The membrane-bound EssB is an integral and essential component of the bacterial type VII secretion system that can contribute to pathogenicity. One of these is EssB, a 50-kDa bitopic integral membrane protein that is conserved among T7SS gene clusters in Firmicutes. The architecture of Geobacillus thermodenitrificans EssB has been investigated by combining crystallographic and EPR spectroscopic methods. The protein forms a dimer that straddles the cytoplasmic membrane.

We determined the crystal structure of EssB-N using a construct comprising the entire predicted cytoplasmic fragment (Ser2 to Asp214). The structure of EssB-N was determined at 1.7 Å resolution. The asymmetric unit consists of a single polypeptide folded into an elongated structure, approximately 55 Å long and 35 Å wide, which consists of two domains. The N-terminal domain is dominated by a four-stranded antiparallel β sheet. The C-terminal domain consists of a helical bundle formed by two antiparallel helix pairs, α4/α5 and α7/α8. A cleft, approximately 30 Å deep, is formed between the two domains, blocked at one side by the interdomain connecting loop that links β4 to β5. The EssB-N segment resembles the bilobal structure of ATP-dependent protein kinases, i.e., an N-terminal domain or N-lobe with a β sheet packed against an intersecting α-helix, and a predominantly α-helical C-terminal domain (C-lobe; Zoltner et al., 2013). An overlay provides a Z-score of 10.4 and a root-mean-square deviation (rmsd) of 4.4 Å for an alignment of 173 Cα-atoms. These values suggest a distant evolutionary relationship but the catalytic residues are absent from EssB-N. However, at the C-terminal inner surface of the EssB cleft, as well as at the domain contact area, a remarkable degree of structural similarity is evident (Zoltner et al., 2013). The transition to a monomeric state appears to be influenced by a combination of low pH and high ionic strength, which matches the crystallization conditions used for EssB-N where we may have been selecting out the monomer.

> GASTSEKKTYLETQLDAVMINDQPYTVIFQRAKLKMQDPLELEVLKEVDPCIVRDIDVSEDEVKVVIKPPSSFLTFAAIRKTTLLSRIRAAIHLVSKVKHHSARRLIFIVCPENLMFNRALEPFFLHVGVKESLPPDEWDDERLLREVKATVLALTEGEYRFDEYLKFHETLKCSPIAKELWQADHLDAVLAVLEKWVDEEEAKERAKVHIPKKRWNMQ>[4x]MKRLEGKVAIVTSSTRGIGRASAEALAKEGALVYLAARSEELANEVIADIKKQGGVAKFVYFNAREEETYTSMVEKVAEAEGRIDILVNNYGGTNVNLDKNLTAGDTDEFFRILKDNVQSVYLPAKAAIPHMEKVGGGSIVNISTIGSVVPDISRIAYCVSKSAINSLTQNIALQYARKNIRCNAVLPGLIGTRAALENMTDEFRDSFLGHVPLNRVGRPEDIANAVLYYASDDSGYVTGMIHEVAGGFALGTPQYSEYCPR

7α-hydroxysteroid dehydrogenases (7α-HSDH) is responsible for reversibly catalysing the oxidation of C7 α-oriented hydroxyl of the steroid nucleus in the bile acid metabolism and has been detected in numerous genera of bacteria and in mammal. To date, three-dimensional structures of two 7α-HSDHs from Escherichia coli and Brucella Melitensis have been determined, and the characteristics of folding pattern in both the two 7α-HSDHs indicate that they belong to the short-chain dehydrogenases/reductases (SDRs), whose members are dimeric or tetrameric and generally share low sequence identity possessing a single-domain globular Rossmann-related fold. As one of the SDRs, with the similar structure to the two 7α-HSDHs above, CA 7α-HSDH possesses the typical Rossmann-fold that each monomer consists of seven parallel β-strands as a core (β-sheet core) and α-helices located between β-strands at the surface of the globular molecules. Nevertheless, differing from EC 7α-HSDH, CA 7α-HSDH is NADP(H)-dependent and has a more complex C-terminal structure.

To unravel the NADP(H) recognition in 7α-HSDH, we determined the crystal structure of CA 7α-HSDH complexed with NADP+ and taurochenodeoxycholic acid (TCDCA) at resolution 2.0 Å. The three-dimensional structure of CA 7α-HSDH complexed with NADP+ and TCDCA belonged to the P212121 space group and was determined at resolution of 2.0 Å by the molecular displacement method and refined to crystallographic R-factor of 0.182 (Rfree = 0.222). An asymmetric unit of CA 7α-HSDH crystal structure includes four subunits. However, CA 7α-HSDH possesses the active site, Thr145-Tyr158-Lys162, rather than Ser-Tyr-Lys triad. The residue Thr145 forms hydrogen bond with C7-OH of TCDCA while the residue Lys162 forms hydrogen bonds with 2′- and 3′-hydroxyl group of the nicotinamide ribose moiety in NADP+. The phenolic hydroxyl of Tyr158 form hydrogen bonds with C7-OH of TCDCA and 2′-hydroxyl group of the nicotinamide ribose of NADP+. Thr15, Arg16, Arg38 and Arg194 formed a positive charge-rich environment surrounding the 2′-phosphate of adenine ribose and these residues determined the cofactor specificity in CA 7α-HSDH. Furthermore, the amino groups in Arg16, Arg38 and Arg194 form strong hydrogen bonds with the oxygen atoms in the 2′-phosphate of adenine ribose of NADP+. Especially, the nitrogen atom in guanidinium of Arg38 is close (~4 Å) to the adenine ring of NADP+ forming the cation-π stacking. Significantly, we captured an active state of the coenzyme NADP+ with the rather weak electron density of the nicotinamide moiety, which confirmed that nicotinamide moiety of NADP+ act as electron carrier in the dehydrogenation reaction.2,4-DIAMINO-6-[2,3-DIHYDROXY-PROP-3-YL]-5,6,7,8-TETRAHYDROPTERIDINE 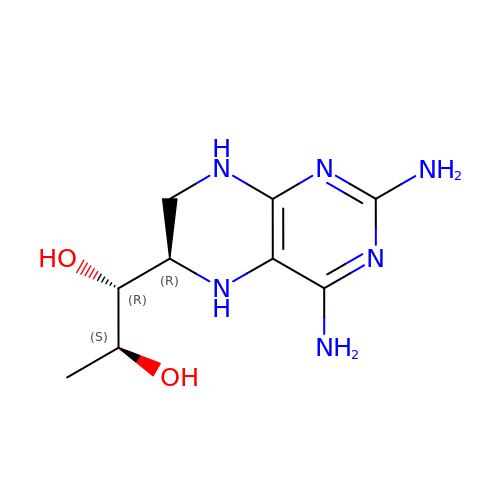| C9 H16 N6 O2 | NDSDGUULXHNXGA-RPDRRWSUSA-N>GAMADKNAKNENGDNEKGKKKNNAQNKNAQKKKVEEPKNLDDITRLNIIVGYVEEVEIHPDADTLYCLKINVGEEKSRDICSGLRLKKNSEDLLHKYVLVLANLKEKSLRGRKSHGMVLCGSFGEQIELLAPPDGVNVGERIICENMDVNKLPDKTLSFDKEKNPFFHIQPHLLVKNGVAHYKDAKWLSSKGEITC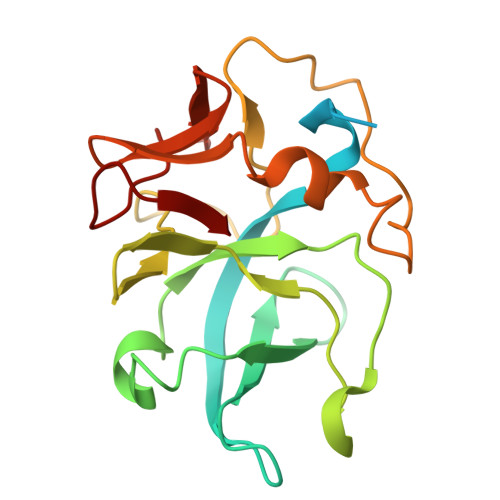PLEQGTIS[2x]UvrD is classified as a SF1A helicase and plays important functions in DNA replication, recombinational repair, methyl-directed mismatch repair and nucleotide excision repair. UvrD consists of two RecA-like domains (1A and 2A) that are responsible for nucleotide binding and hydrolysis and two additional domains (1B and 2B) that are involved in dsDNA binding. Here we present crystal structures of full-length and a C-terminally truncated construct of D. radiodurans UvrD (drUvrD) in complex with 3′-tailed dsDNA. Our structures obtained in apo- and AMPPNP bound states provide us with several snapshots of this essential cellular process and reveal a large-scale spiral movement of UvrD around the duplexed DNA.

Crystals containing the C-terminally truncated drUvrD∆C, an 18-mer DNA duplex with 7nt ssDNA extensions at its 3′-ends and AMPPNP diffracted to higher resolution. This complex produced two crystal forms (I and II) diffracting respectively to 2.5 and 3.0 Å resolution. Crystal form I appeared very rapidly (<1 day) and belonged to space group P212121 with two protein monomers and one DNA duplex per asymmetric unit, while crystal form II appeared after at least one week and belonged to space group P21 with four molecules of protein and two DNA duplexes per asymmetric unit. In both drUvrDFL and drUvrD∆C form I, the two drUvrD protomers are located on the same side of the DNA duplex and induce a bend in the DNA. In drUvrD∆C form I, four nucleotides (nt21-24) are tightly bound in the ssDNA-binding pocket. The terminal nucleotide (nt25) has already exited the helicase and is no longer visible in the electron density maps. Nucleotides 21 and 22 interact with Arg362 and Asn364 (motif IVa) and stack against Phe263 (motif III) that interferes with the regular stacking of the ssDNA bases and forces nucleotides 23 and 24 to adopt an orientation orthogonal to nucleotides 21 and 22. Nucleotide 24 is stabilized in this conformation by π-stacking of the base between Arg264 and Phe196 (motif Id) and of the deoxyribose ring against Phe65 (motif Ia). In form I, the third binding site involves Arg459 from the α19-α20 HLH motif, which interacts with the deoxyribose ring of nt13 (opposite strand) in the minor groove of the DNA duplex, while in form II, Phe633 from the β-hairpin motif stacks against the first base-pair (nt1=nt18) of the duplex. In drUvrD∆C form I and drUvrDFL, the nucleotides at the junction between the dsDNA and the ssDNA are poorly defined, indicating that this region is relatively flexible.

>[2x]MTSSAGPDLLQALNPTQAQAADHFTGPALVIAGAGSGKTRTLIYRIAHLIGHYGVHPGEILAVTFTNKAAAEMRERAGHLVPGAGDLWMSTFHSAGVRILRTYGEHIGLRRGFVIYDDDDQLDIIKEVMGSIPGIGAETQPRVIRGIIDRAKSNLWTPDDLDRSREPFISGLPRDAAAEAYRRYEVRKKGQNAIDFGDLITETVRLFKEVPGVLDKVQNKAKFIHVDEYQDTNRAQYELTRLLASRDRNLLVVGDPDQSIYKFRGADIQNILDFQKDYPDAKVYMLEHNYRSSARVLEAANKLIENNTERLDKTLKPVKEAGQPVTFHRATDHRAEGDYVADWLTRLHGEGRAWSEMAILYRTNAQSRVIEESLRRVQIPARIVGGVGFYDRREIRDILAYARLALNPADDVALRRIIGRPRRGIGDTALQKLMEWARTHHTSVLTACANAAEQNILDRGAHKATEFAGLMEAMSEAADNYEPAAFLRFVMETSGYLDLLRQEGQEGQVRLENLEELVSAAEEWSQDEANVGGSIADFLDDAALLSSVDDMRTKAENKGAPEDAVTLMTLHNAKGLEFPVVFIVGVEQGLLPSKGAIAEGPSGIEEERRLFYVGITRAMERLLMTAAQNRMQFGKTNAAEDSAFLEDIEGLFDTVDPYGQPIEYR>[3x]GS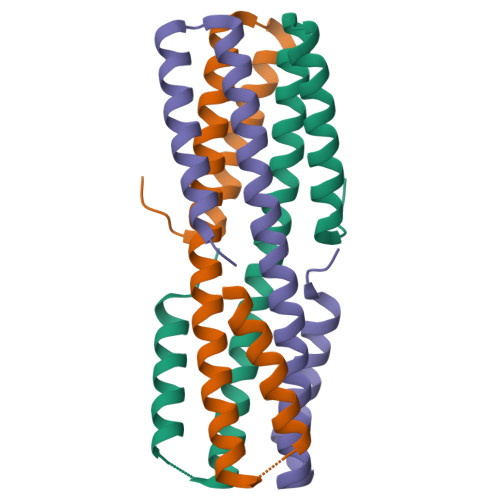HMGTEDLKYSLERLREILERLEENPSEKQIVEAIRAIVENNAQIVEAIRAIVENNAQIVEILRAIIEALEAIGGGTKILEEMKKLLKDLKRSLERG> MNAHLANEVQYDLGHGPGRPSSLVHVIISSECLAAAGIPLAALMRGRPGLGTAANFQVEIQTRAHATGDCTPWCTAFAAYVPADAVGELLAPVVPAHPGLLPRASSAGGLFVSLPVVCDAQGVYDPYAVAALRLAWGSGASCARVILFSYDELVPPNTRYAADSTRIMRVCRHLCRYVALLGAAAPPAAKEAAAHLSMGLGESASPRPQPLARPHAGAPADPPIVGASDPPISPEEQLTAPGGDTTAAQDVSIAQENEEILALVQRAVQDVTRRHPVRARTGRAACGVASGLRQGALVHQAVSGGAMGAADADAVLAGLEPPGGGRFVAPAPHGPGGEDILNDVLTLTPGTAKPRSLVEWLDRGWEALAGGDRPDWLWSRRSISVVLRHHYGTKQRFVVVSYENSVAWGGRRARPPLLSSALATALTEACAAERVVRPHQLSPAGQAELLLRFPALEVPLRHPRPVLPPFDIAAEVAFTARIHLACLRALGQAIRAALQGGPRISQRLRYDFGPDQRAWLGEVTRRFPILLENLMRAVEGTAPDAFFHTAYALAVLAHLGGRGGRGRRVVPLGDDLPARFADSDGHYVFDYYSTSGDTLRLNNRPIAVAMDGDVSKREQSKCRFMEAVPSTAPRRVCEQYLPGESYAYLCLGFNRRLCGIVVFPGGFAFTINIAAYLSLSDPVARAAVLRFCRKVSS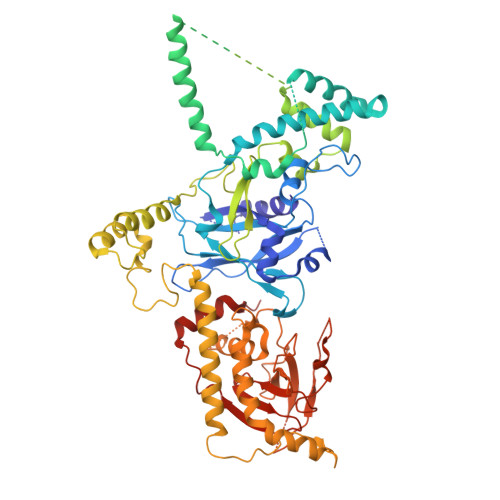GNGRSR> MDKFRVQ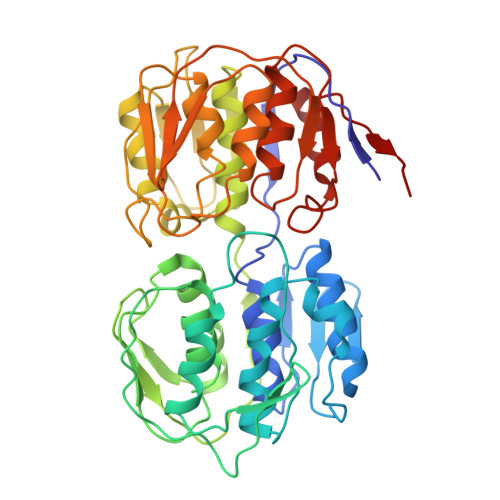GPTKLQGEVTISGAKNAALPILFAALLAEEPVEIQNVPKLKDVDTSMKLLSQLGAKVERNGSVHIDARDVNVFCAPYDLVKTMRASIWALGPLVARFGQGQVSLPGGCTIGARPVDLHISGLEQLGATIKLEEGYVKASVDGRLKGAHIVMDKVSVGATVTIMCAATLAEGTTIIENAAREPEIVDTANFLITLGAKISGQGTDRIVIEGVERLGGGVYRVLPDRIETGTFLVAAAISRGKIICRNAQPDTLDAVLAKLRDAGADIEVGEDWISLDMHGKRPKAVNVRTAPHPAFPTDMQAQFTLLNLVAEGTGFITETVFENRFMHVPELSRMGAHAEIESNTVICHGVEKLSGAQVMATDLRASASLVLAGCIAEGTTVVDRIYHIDRGYERIEDKLRALGANIERVKGE>[2x]MCKDKNEKKNYEHVNANEKNGYLASEKNELTKNKVEEHTYDYDYVVIGGGPGGMASAKEAAAHGARVLLFDYVKPSSQGTKWGIGGTCVNVGCVPKKLMHYAGHMGSIFKLDSKAYGWKFDNLKHDWKKLVTTVQSHIRSLNFSYMTGLRSSKVKYINGLAKLKDKNTVSYYLKGDLSKEETVTGKYILIATGCRPHIPDDVEGAKELSITSDDIFSLKKDPGKTLVVGASYVALECSGFLNSLGYDVTVAVRSIVLRGFDQQCAVKVKLYMEEQGVMFKNGILPKKLTKMDDKILVEFSDKTSELYDTVLYAIGRKGDIDGLNLESLNMNVNKSNNKIIADHLSCTNIPSIFAVGDVAENVPELAPVAIKAGEILARRLFKDSDEIMDYSYIPTSIYTPIEY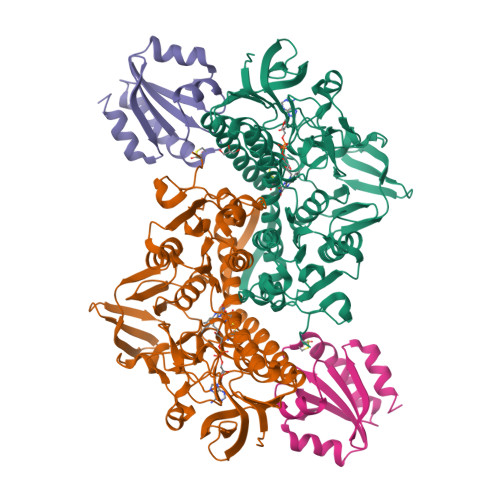GACGYSEEKAYELYGKSNVEVFLQEFNNLEISAVHRQKHIRAQKDEYDLDVSSTCLAKLVCLKNEDNRVIGFHYVGPNAGEVTQGMALALRLKVKKKDFDNCIGIHPTDAESFMNLFVTISSGLSYAAKGGCGGGKSG;>[2x]RGSHHHHHHGSVKIVTSQAEFDSIISQNELVIVDFFAEWCGPSKRIAPFYEECSKTYTKMVFIKVDVDEVSEVTEKENITSMPTFKVYKNGSSVDTLLGANDSALKQLIEKYAA>DNINTLWTGVNPTEANCQIMNSSESNDCKLILTLVKTGALVTAFVYVIGVSNNFNMLTTHRNIN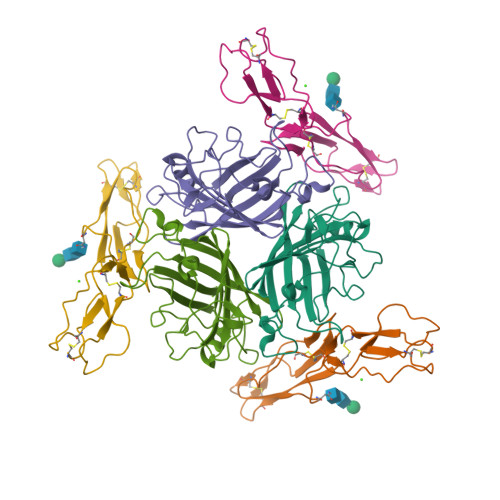FTAELFFDSTGNLLTRLSSLKTPLNHKSGQNMATGAITNAKGFMPSTTAYPFNDNSREKENYIYGTCYYTASDRTAFPIDISVMLNRRAINDETSYCIRITWSWNTGDAPEVQTSATTLVTSPFTFYYIREDD[2x];>[2x]CEEPPTFEAMELIGKPKPYYEIGERVDYKCKKGYFYIPPLATHTICDRNHTWLPVSDDACYRETCPYIRDPLNGQAVPANGTYEFGYQMHFICNEGYYLIGEEILYCELKGSVAIWSGKPPICEKV> GGLEKDFLPLYFGWFLTKKSSETLRKAGQVFLEELGNHKAFKKELRHFISGDEPKEKLELVSYFGKRPPGVLHCTTKFCDYGKAAGAEEYAQQEVVKRSYGKAFKLSISALFVTPKTAGAQVVLTDQELQLWPSDLDKPSASEGLPPGSRAQVTLGCAADVQPVQTGLDLLDILQQVKGGSQGEAVGELPRGKLYSLG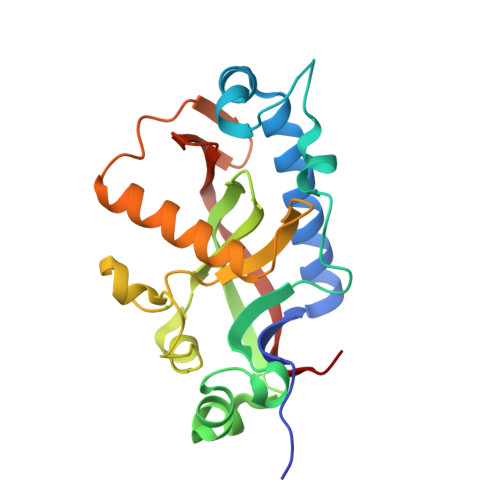KGRWMLSLTKKMEVKAIFTGYYG>MSLSDDIKVLGISGSLRSGSYNSAALQEAIGLVPPGMSIELADISGIPLYNEDVYALGFPPAVERFREQIRAADALLFATPEYNYSMAGVLKNAIDWASRPPEQPFSGKPAAILGASAGRFGTARAQYHLRQTLVFLDVHPLNKPEVMISSAQNAFDAQGR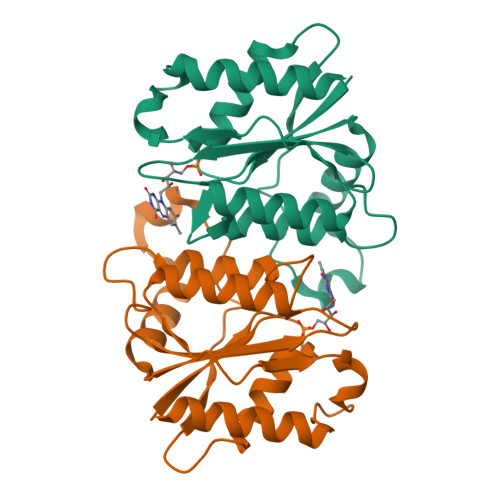LLDDKARELIQQQLQALQLWVREGGSHHHHHH[2x]N'-[(1S,2R)-2-[(2R,4S)-4-benzylpiperidin-2-yl]-1-(3,5-difluorobenzyl)-2-hydroxyethyl]-5-methyl-N,N-dipropylbenzene-1,3-dicarboxamide 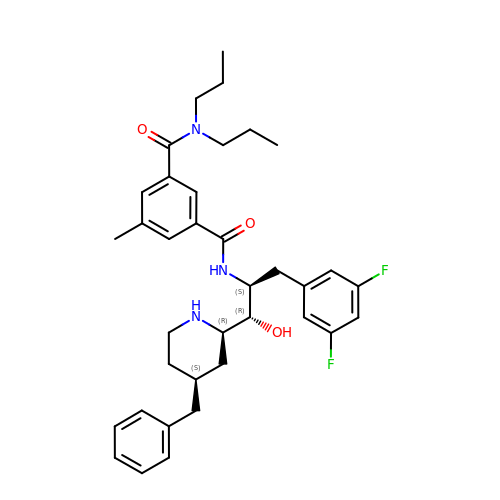| C36 H45 F2 N3 O3 | UKXYKYZOSFWZIM-FLQGXGFZSA-N The IRES from encephalomyocarditis virus (EMCV) interacts with eukaryotic translation initiation factor 4 G (eIF4G), recruiting the ribosomal subunit for translation. Within the EMCV IRES, the region G680-C787, designated as J-K-St in this study, is responsible for the specific capture of the eIF4GHEAT1. We previously determined the structure of this J-K-St region by solution NMR spectroscopy. It is composed of two stem-loops (J and K domains) bifurcating from a base stem (St domain). At the three-way junction, a highly conserved sequence of six adenosines forms a short stem loop, termed ASL, which interacts with the J, K, and St domains at the junctional part.

Further local refinement with a mask on J-K-St/eIF4GHEAT1 yielded the focused cryo-EM map of the region at a resolution of 3.7 Å. Here, in the cryo-EM structure at 3.7 Å resolution, we clearly showed that J-K-St binds to eIF4GHEAT1 via the J and St domains by adjusting their relative angles to adhere to the surface of eIF4GHEAT1, but not significantly changing the overall structure of eIF4GHEAT1. In the J domain, G702, U703, A704, C705, U722, G723, A724, and U725 interact with eIF4GHEAT1 from the minor groove side. All of these bases, except for A724, interact mainly with the positively charged patch on eIF4GHEAT1 including side chain atoms of Arg 840, Lys841, Lys922, Lys925, and Arg954, whereas the nucleobase of A724 is extruded from the stem to deeply interact with the negatively charged cleft including sidechain atoms of Asp918. In the St domain, G690, A691, U692, G693, C776, G777, U778, and C779 also interact with eIF4GHEAT1 from the minor groove side. All of these residues, except for G777, interact mainly with the positively charged patch on the eIF4GHEAT1 including sidechain atoms of Lys826 and Asn838, whereas the nucleobase of G777 is extruded from the stem to interact with another negatively charged cleft including the mainchain carboxy atoms of Thr784, Leu786, and Ala824, which differs from that contacted by the J domain. Since the cavity on the St domain formed by extrusion of G777 was filled by a lysine residue, Lys826, of eIF4GHEAT1, the flipping-out of G777 is important not only for its direct interaction with eIF4GHEAT1, but also for the formation of the binding pocket for this basic residue. In the J-K-St structure in complex with eIF4GHEAT1/eIF4A, the ASL domain does not form the short stem-loop, and the upper stem of the St domain, which includes the eIF4GHEAT1-binding site, exhibits large base-pairing rearrangements within the ASL domain bases; i.e., G686-A781, A687-U780, G689-C779, G690-U778, A691-C776, U692-A774, and G683-A773. G777 is flipped out to interact with the cleft of eIF4GHEAT1.

> MNHKVHHHHHHIEGRHMELGTLEDRGEEDADGSKTQDLFRRVRSILNKLTPQMFQQLMKQVTQLAIDTEERLKGVIDLIFEKAISEPNFSVAYANMCRCLMALKVPTTEKPTVTVNFRKLLLNRCQKEFEKDKDDDEVFEKKQKEMDEAATAEERGRLKEELEEARDIARRRSLGNIKFIGELFKLKMLTEAIMHDCVVKLLKNHDEESLECLCRLLTTIGKDLDFEKAKPRMDQYFNQMEKIIKEKKTSSRIRFMLQDVLDLRGSNWVP>YVDKKAREYAQDALKFIQRSGSNFLACKNLKERLENNGFINLSEGETWNLNKNEGYVLCKENRNICGFFVGKNFNIDTGSILISIGHIDSCALKISPNNNVIKKKIHQINVECYGSGLWHTWFDRSLGLSGQVLYKKGNKLVEKLIQINKSVLFLPSLAIHLQNRTRYDFSVKINYENHIKPIISTTLFNQLNKCKRNNVHHDTILTTDTKFSHKENSQNKRDDQMCHSFNDKDVSNHNLDKNTIEHLTNQQNEEKNKHTKDNPNSKDIVEHINTDNSYPLLYLLSKELNCKEEDILDFELCLMDTQEPCFTGVYEEFIEGARFDNLLGSFCVFEGFIELVNSIKNHTSNENTNHTNNITNDINDNIHNNLYISIGYDHEEIGSLSEVGARSYCTKNFIDRIISSVFKKEIHEKNLSVQEIYGNLVNRSFILNVDMAHCSHPNYPETVQDNHQLFFHEGIAIKYNTNKNYVTSPLHASLIKRTFELYYNKYKQQIKYQNFMVKNDTPCGSTVGSMVAANLSMPGIDIGIPQLAMHSIREIAAVHDVFFLIKGVFAFYTYYNQVL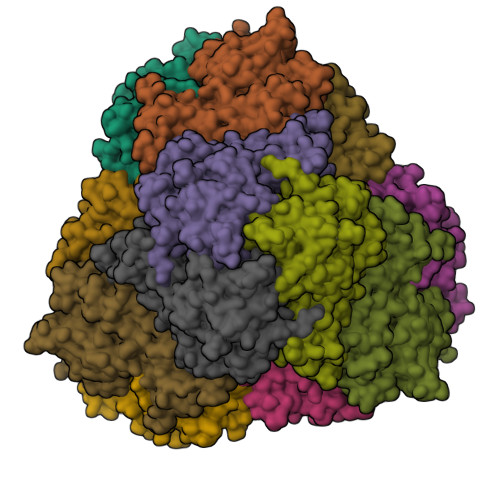STCVHDK[4x]> MAESTTLETIEIHPITFPPEVLARISPELSLQRHLSLGIR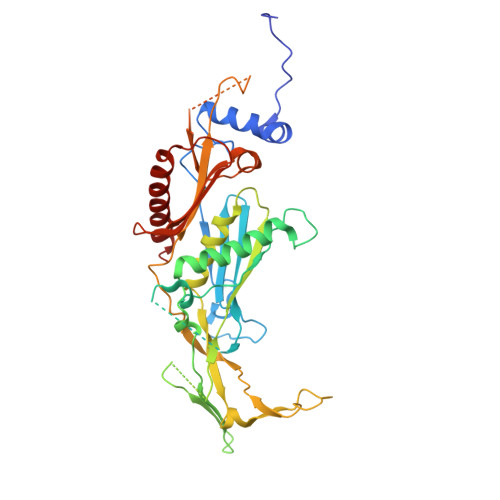PCLRKYEEFRDVAIENNTLSRYADAGNIDTKNNILGSNVLKSGKTIVITSITGGIIEETSAAIKDLDDFGEEELFEVTKEEDIIANYASVYPVVEVERGRVGACTDEEMTISQKLHDSILHSRILPKKALKVKAGVRSANEDGTFSVLYPDELEDDTLNETNLKMKRKWSYVLYAKIVVLSRTGPVFDLCWNSLMYALQSVKLPRAFIDERASDLRMTIRTRGRSATIRETYEIICDQTKSVPLMINAKNIAFASNYGIVELDPECQLQNSDNSEEEEVDIDMDKLNTVLIADLDTEAEETSIHSTISILAAPSGNYKQLTLMGGGAKITPEMIKRSLLLSRVRADDLSTRFNI>[2x]MKQIYDTLQLIPVDKIDLHEAFEPSRLEKTKESIA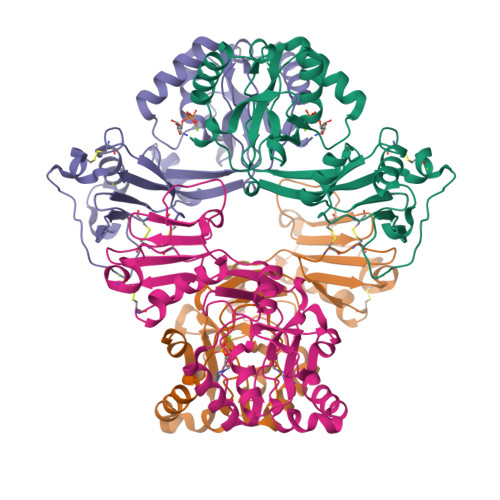KEQHLRHPVLVVKTLFGRYMVIDGVHRFMSLKALGCEVIPVQVIQRTQYSIGSWHHKIPNGAWCEGLTDEELLPWTTEVRDETPFITMCDQQTEHYLYAADLTADKLDVWKKVVNSYSASCNVERVPHSACLCLDSNDILMKYQPLQIGEIEAVVQRGQTVPAGVTRFNIAGRCLNLQVPLHLLKNSNLGNQEQWHTFLQKKIESMRCYTEKIYLIEAE Biuret hydrolase (BiuH) hydrolyzes biuret to allophanate and is part of the Isochorismatase-like hydrolase (IHL) protein family within the cysteine hydrolase superfamily. TrtA is a member of the isochorismatase-like hydrolase (IHL) protein family, similarly to BiuH, and has a catalytic efficiency (kcat/KM) of 6 x 105 M−1s−1, a KM for triuret of 20 μM, and exquisite substrate specificity. TrtA and BiuH are members of the IHL protein family that possess the catalytic triad comprised of a cysteine, aspartate, and lysine residue. Interestingly, the active sites of TrtA and BiuH are almost identical in sequence, and so it was hypothesized that triuret is the substrate for TrtA, funneling into biuret metabolism.

The triuret hydrolase (trtA) gene (NCBI accession number PKOI01000001.1) tested in this study comes from Herbaspirillum sp. BH-1, which was isolated from a biuret-fertilized potato field. To remove a possible intrinsically disordered region, a C-terminal deletion was made for crystallographic purposes. TrtA elutes as a dimer by size-exclusion chromatography, and the monomer adopts a fold typical of the IHL protein family with six parallel β-strands alternating with six α-helices (Rossmann-like) in addition to a two-strand antiparallel β-sheet at the N-terminus. Helices α6 and α7 provide most of the interactions between the two subunits in the dimer while α4 also has some contact at this interface. The α2 helix shows the highest mobility as illustrated by high B-factor values in the apo crystal and undergoes a significant conformational change (∼4.5 Å) when triuret or biuret is bound in the active site. The catalytic triad that has been previously defined in the cysteine hydrolase superfamily is present in TrtA. It is represented by residues D24, K129, and C162. Also present in TrtA is a cis-peptide bond in the active site between residues V157 and T158, which is signature of the IHL protein family. In the apo WT structure, beta-mercaptoethanol (BME) was found covalently attached to the catalytic cysteine of every subunit. The other chains in the biuret cocrystal that do not have biuret bound, as well as the apo WT crystal, are in the open conformation.

>GSHMIRIDATPYPYQFHPRSTALVVIDMQRDFIEEGGFGSALGNDVRPLAAIVPTVAALLQLAREAGMLVVHTRESHLPDLSDCPRSKRLRGNPTLGIGDVGPMGRILVQGEPGNQILPQLAPVEGELVIDKPGKGAFYATDLHAQLQERRITHLLVAGVTTEVCVQTSMREANDRGYECLVIEDACASYFPDFHRITLEMLTAQGGIVGWRTPLAQLQAGVA[8x]2-[(1R)-3-amino-1-phenyl-propoxy]-4-chloro-benzonitrile | 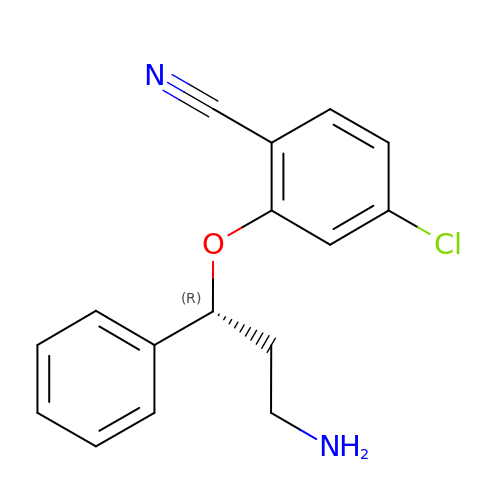C16 H15 Cl N2 O | GPCXUXJZOSOVLY-OAHLLOKOSA-N> AGPVTWVMMIACVVVFIAMQILGDQEVMLWLAWPFDPTLKFEFWRYFTHALMHFSLMHILFNLLWWWYLGGAVEKRLGSGKLIVITLISALLSGYVQQKFSGPWFGGLTGVVYALMGYVWLRGERD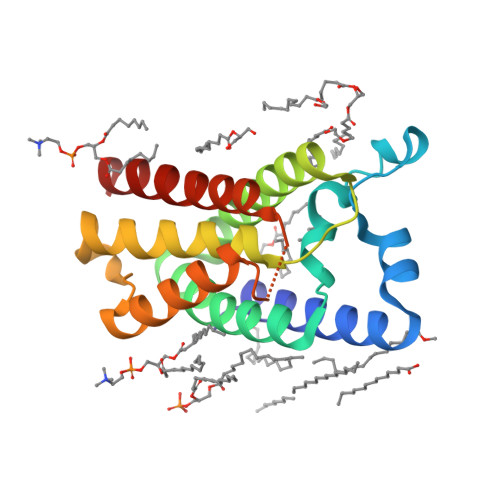PQSGIYLQRGLIIFALIWIVAGWFDLFGMSMANGAHIAGLAVGLAMAFVDSLNA>MSSRSELLLEKFAEKIGIGSISFNENRLCSFAIDEIYYISLSDANDEYMMIYGVCGKFPTDNSNFALEILNANLWFAENGGPYLCYEAGAQSLLLALRFPLDDATPEKLENEIEVVVKSMENLYLVLHNQGITLENEHMKIEEISSSDNKHYYAGR[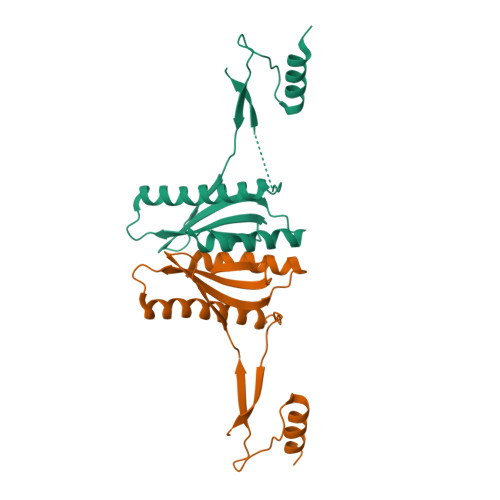2x]3-{[(4-chlorophenyl)carbamoyl]amino}benzoic 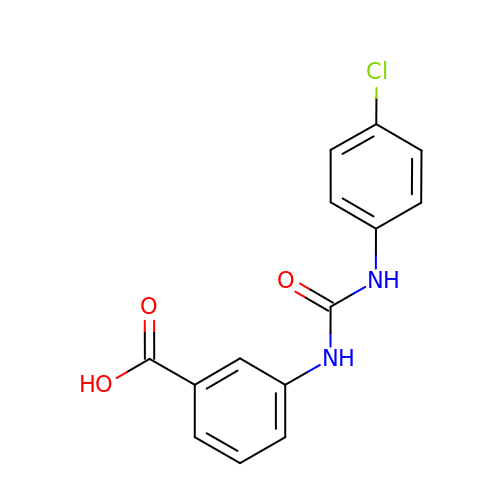acid | C14 H11 Cl N2 O3 | QZVLALCHSFACLK-UHFFFAOYSA-N>[2x]MAKDKEFQV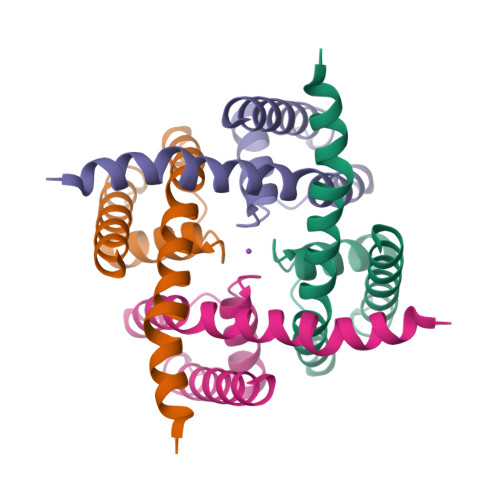LFVLTILTLISGTIFYSTVEGLRPIDALYFSVVTLTTVGETPTPQTDFGKIFTILYIFIGIGLVFGFIHKLAVNVQLPSILSNLVPRG>MASHHHHHHHENLYFQGMSGIQTVSKSATDLTEMVKKITTMNRGEFRQITLATGAGKTTELPRSVIEEIGRHKRVLVLIPLRAAAESVYQYMRQKHPSIAFNLRIGEMKEGDMATGITYASYGYFCQMSQPKLRAAMVEYSFIFLDEYHCATPEQLAIMGKIHRFSENLRVV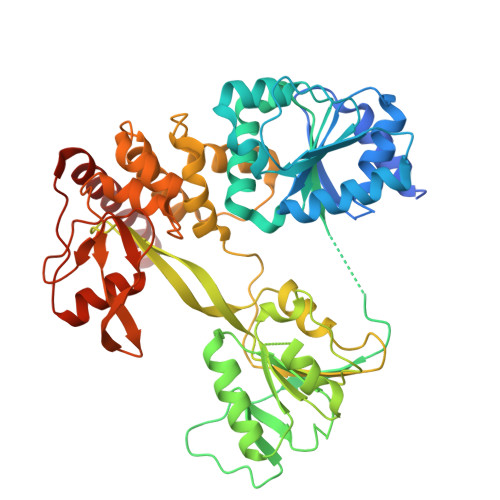AMTATPAGTVTTTGQKHPIEEFIAPEVMKGEDLGSEYLDIAGLKIPVEEMKNNMLVFVPTRNMAVEAAKKLKAKGYNSGYYYSGEDPSNLRVVTSQSPYVVVATNAIESGVTLPDLDVVVDTGLKCEKRIRLSPKMPFIVTGLKRMAVTIGEQAQRRGRVGRVKPGRYYRSQETPVGSKDYHYDLLQAQRYGIEDGINITKSFREMNYDWSLYEEDSLMITQLEILNNLLISEELPMAVKNIMARTDHPEPIKLAYNSYETQVPVLFPKIRNGEVTDTYDNYTFLNARKLGDDVPPYVYATEDEDLAVELLGLDWPDPGNQGTVEAGRALKQVVGLSTAENALL[4x]> PGN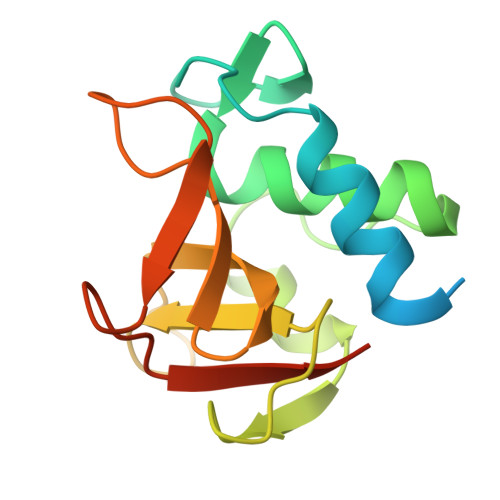STGSNATNNTTNTTPTPTPSGSVNGAAIVAEAYKYIGTPYVWGGKDPSGFDCSGFTRYVYLQVTGRDIGGWTVPQESAGTKISVSQAKAGDLLFWGSPGGTYHVAIALGGGQYIHAPQPGESVKVGSVQWFAPDFAVSMLEHHHHHH>MHGTTRTPAARRRLSAIGAAVALAAGMLVALGAPTAQAAPAAQAAPAAQAATAGADLPFTSVEAESATTTGTKIGPDYTQGTLASEASGRQAVRLDAGQRVEFTVPRAANALTVAYSVPDGQSGTLDVYVNGTKLDRSLTVTSKYSYVDTGWIPGAKTHHFYDNTRLLLGRDVQAGDTVTLQATNVQVTVDVADFEQVSAAAGQPAGSVSVTDKGADPTGQGDSTQAFRDAIAAAQGGVVWIPPGDYRITGPLSGVQNVTLQGAGSWYSVVHSSHFIDQTDSAGHVHLKDFAVIGEVTERVDSSPDNFVNGSLGPGSSVSGMWIQHV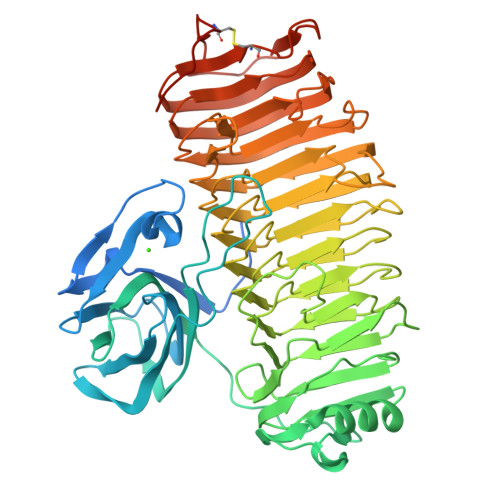KVGLWLTGTNDDLVVENNRILDTTADGLNLNGTAKNVTVRDNFLRNQGDDALAMWSLYAPDTDCRFENNTITQPNLANGIAIYGGTDITVKGNLISDTNALGSGIAISNQKFAEPFHPLAGTITVDGNTLVRTGAINPNWNHPMGALRVDSYDSAIEARVDITDTTITDSPYSAFEFVSGGGQGHAVKNVTVDGAAVKNTGTVVVQAEAPGEATFRNVTATGTGAAGIYNCPFPSGSGTFTVTDGGGNSGWDTTWSDCSTWPQPGQGNPEKLAAALEHHHHHH[2x]>[2x]MASLNEHEGEVAYDKKEDAEISMHMNEQDKLDVPSLVEICKQQLIVILKDMCADSNSSDEKASFMYHLNRLRSAVTVVDLHNYIA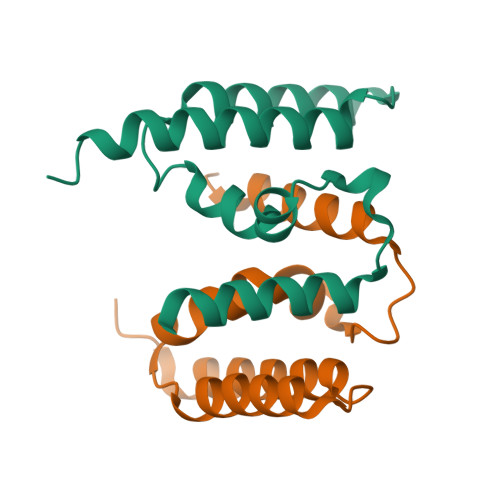VFGPCLSYNKLPSTWNISVCDYLKQQLNILRAADSQQSSSNHVSYLELHNDYEDIIHDKKGNATTTASNSMQGNMNSNNLNSQLSMKGSSIHMNSANSTSNVSGNATGNASGHISINWSHPQFEK> FNYKPTPWTRADALKVHSDDPTTTQPLVDVAFPVMSEEVFIWDTMPLRDFDGDIVSVNGWCVIFTLTADRNTNNPDFQDENGNYDIKRDWEDRHGRARICYWYSRTGKDWIFGGRVMAEGVSPTTREWAGTPILLNDEGDIDLYYTCVTPGATIAKVRGKIVTSDEGVSLEGFQHVKSLFSADGKIYQTEEQNAYWNFRDPSPFIDKNDGKLYMLFEGNVAGSRGTHEITQEDMGSVPPGYENVGGARYQVGCIGLAVAKDLSGDEWEILPPLITAVGVNDQTERPHFVFQEGKYYLFTISHKYTFADNL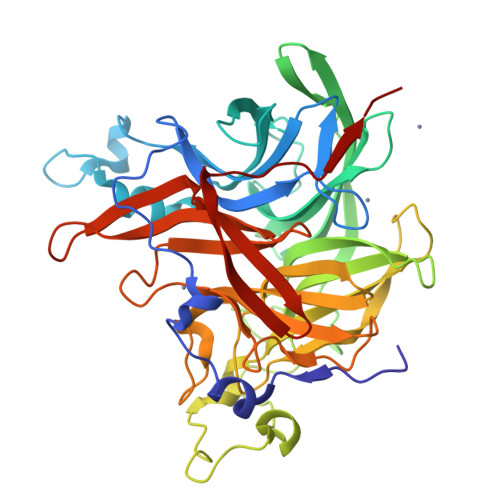TGPDGVYGFVSNQLTGPYTPMNSSGLVLGNPSSQPFQTYSHYVMPNGLVTSFIDSVPWEGEKFRIGGTEAPTVKILLKGDRSFVVDSFDYGYIPAMKDIILK> MGHHHHHHGSVKIGHYILGDTLGVGTFGKVKVGKHELTGHKVAVKILNRQKIRSLDVVGKIR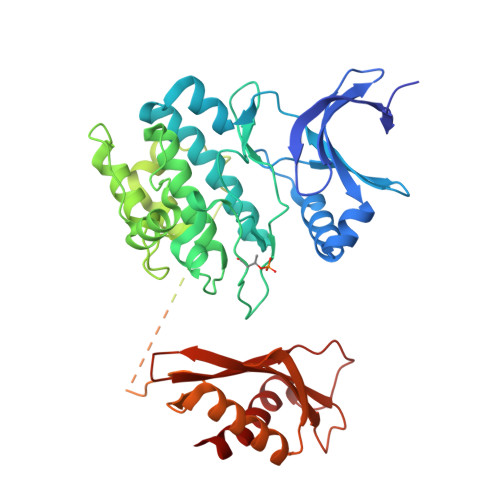REIQNLKLFRHPHIIKLYQVISTPSDIFMVMEYVSGGELFDYICKNGRLDEKESRRLFQQILSGVDYCHRHMVVHRDLKPENVLLDAHMNAKIADFGLSNMMSDGEFLRTSCGSPNYAAPEVISGRLYAGPEVDIWSSGVILYALLCGTLPFDDDHVPTLFKKICDGIFYTPQYLNPSVISLLKHMLQVDPMKRATIKDIREHEWFKQDLPKYLFPEDPSYSSTMIDDEALKEVCEKFECSEEEVLSCLYNRNHQDPLAVAYHLIIDNRRIMNEAKDFYLATSPPDSFLDDHHLTRPHPERVPFLVAETPRARHTLDELNPQKSKHQGVRKAKWHLGIRSQSRPNDIMAEVCRAIKQLDYEWKVVNPYYLRVRRKNPVTSTYSKMSLQLYQVDSRTYLLDFRSIDDELTPRPGSHTIEFFEMCANLIKILAQ INOSITOL-(1,3,4,5)-TETRAKISPHOSPHATE | C6 H16 O18 P4 | 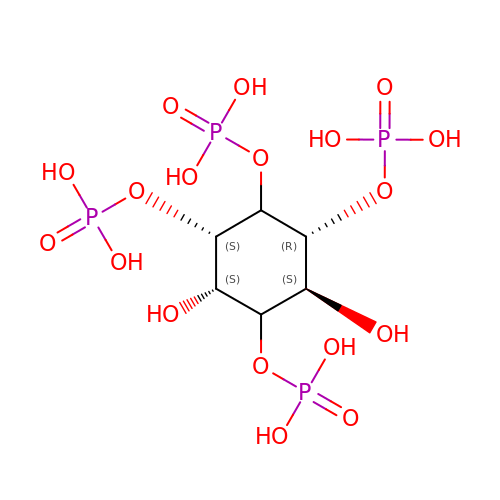CIPFCGZLFXVXBG-CNWJWELYSA-N PREPHENIC 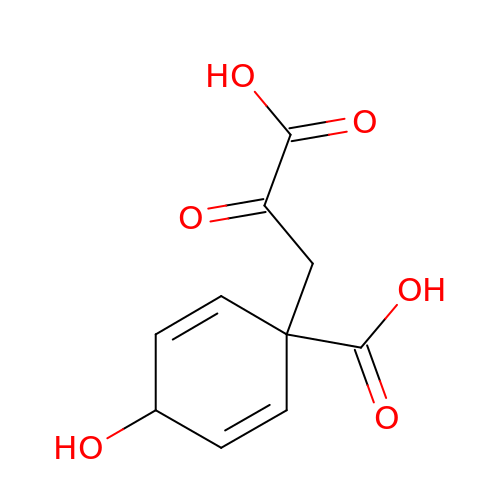ACID | C10 H10 O6 | FPWMCUPFBRFMLH-XGAOUMNUSA-N(5Z)-7-{(1R,4S,5R,6R)-6-[(1E)-oct-1-en-1-yl]-2,3-diazabicyclo[2.2.1]hept-2-en-5-yl}hept-5-enoic acid | C20 H32 N2 O2 | 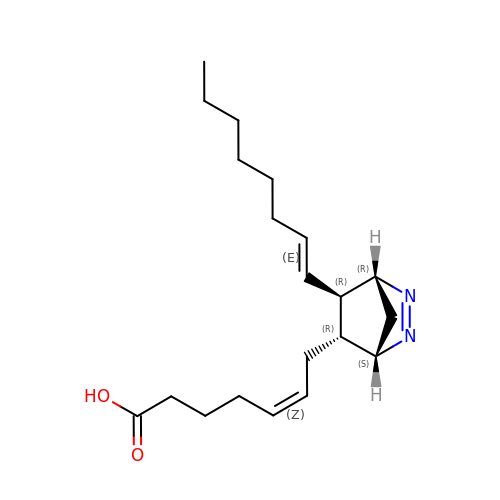SRIZDZJPKIYUPZ-IDUFWMFESA-N> ETGTVPAINYLGAGYDHVRGNPVGDPSSMGDPGIRPPVLRFTYAQNEDGVSNDLTVLQPLGGYVRQYVACRQSETISELSNLSDYQNELSVDASLQGGDPIGLNSFSASTGYRDFAKEVSKKDTRTYMLKNYCMRYEAGVAQSNHFKWNVTLAFAAGVSQLPDVFDAHNPECACSAEQWRQDQNAEACTKTNVPIWISFIEQFGTHFLVRLFAGGKMTYQVTAKRSEVEKMRNMGIDVKTQLKMQLGGVSGGAGQGTSSKKQQSSSEYQMNVQKETLVIGGRPPGQVSDPAALAAWADTVEELPMPVKFEVQPLYHLLPVEKQEAFKQAVTFYSKAVGLTPQDLSALGTKHHHHHH

Toxoplasma and Plasmodium are the parasitic agents of toxoplasmosis and malaria, respectively, and use perforin-like proteins (PLPs) to invade host organisms and complete their life cycles. Escape from the PV, and therefore from the infected cell, for subsequent rounds of infection has been shown to be dependent on the perforin-like protein TgPLP1 (T. gondii PLP). We report structures of the membrane attack complex/perforin (MACPF) and Apicomplexan PLP C-terminal β-pleated sheet (APCβ) domains of TgPLP1. The MACPF domain forms hexameric assemblies, with ring and helix geometries, and the APCβ domain has a novel β-prism fold joined to the MACPF domain by a short linker.

We first obtained oligomeric crystal forms of the TgPLP1 MACPF domain by the use of in situ trypsinization in crystallization drops. On solution of the resulting structures, we found two related assemblies: a ring-shaped hexamer and a helical packing arrangement with six subunits per turn. The helical subunit arrangement was formed in a crystal of space group P65 that diffracted to 2.03 Å with phasing using anomalous scattering from a single platinum derivative. Critically, the helical assembly can only form crystallographically with the trypsinization of TMH2, strongly suggesting that this is an oligomeric form related to that generated following membrane attack by TgPLP1, because cutting away the helical TMH2 will mimic its transition to a β-stranded form. Biologically, no cleavage would occur, but the TMH2 region would move by spontaneous conversion to a membrane-inserted set of β-strands as part of TgPLP1 activity. The orientation of the subunits, with the TMH regions facing inward, is exactly what would be expected for the biological, and usually pore-forming, oligomer formed by MACPF/CDC proteins. We discuss the functional implications of this structure below, but this is the first crystal structure of a MACPF/CDC homo-oligomer in what is likely to reflect a membrane-active, and possibly pore-forming, state. In the crystal structures, all subunit interfaces in the helical assembly are identical, but the ring oligomer has three different interfaces, with three, one, and no main-chain hydrogen bonds, respectively, in contrast to the six in each of the helical subunit interfaces. The subunit interface captured in the helical oligomer could occur in a membrane-bound ring of six subunits, although in solution, it has relaxed into a helical arrangement. In all, these analyses suggest that the interfaces found in the helical assembly are more stable and of biological significance, although the resulting functional oligomer remains to be determined.>MRGSHHHHHHGSMIFDKEDYKAFDPELWNAIDAEAERQQNNIELIASENVVSKAVMAAQGTLLTNKYAEGYPGKRYYGGTAVIDVVETLAIERAKKLFGAKFANVQPHSGSQANAAVYMSLIQPGDTVMGMDLSAGGHLTHGAPVSFSGKTYNFVSYNVDKESELLDYDAILAQAKEVRPKLIVAGASAYSRIIDFAKFREIADAVGAYLMVDMAHIAGLVASGHHPSPVPYAHVTTTTTHKTLRGPRGGLILTDDEDIAKKLNSAVFPGLQGGPLEHVIAAKAVALKEALDPAFKEYGENVIKNAAAMADVFNQHPDFRVISGGTNNHLFLVDVTKVVENGKVAQNVLEEVNITLNKNSIPYEQLSPFKTSGIRVGSPAITSRGMG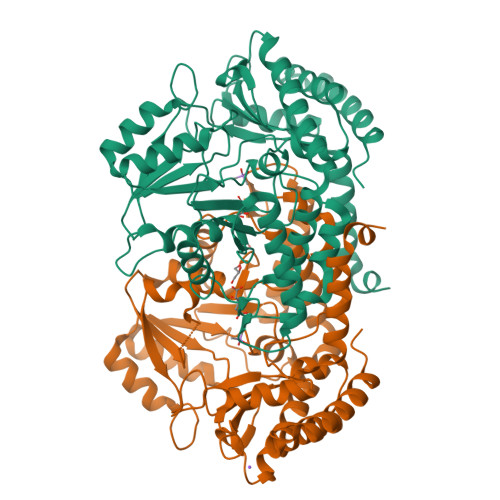EAESRQIAEWMVEALENHDKPEVLERIRGDVKVLTDAFPLY[4x]> AAAAAAAA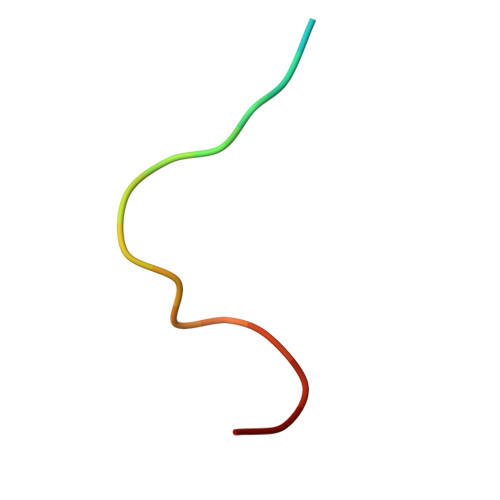AAAAAAAAA> GPGIWLREVDRDKLIAVAKKLKEIIPDRVKGFVVGGKTDDVVATIRDLIALFGPDLEIVVELTELDKAIETMKKAVEAGASAILLRDGVRGVEELRKIAEEAKKLGVKVIVDVTDGPDVLELAREAAALADAIVIDTGLPLDTREAIAALADAAGVDVIFRVSGLDQVDDAVALAARTPAFKGFLLEGVRDVAA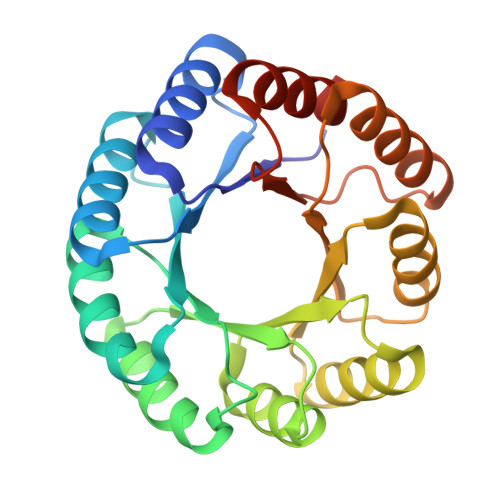AEAVRARLAAAGLTDLDFLLALDGLDVDTAIAAALALLEHHHHHH>[2x]MSYKLTYFPIRGLAEPIRLVLVDQGIKFTDDRINASDWPSMKSHFHFGQLPCLYDGD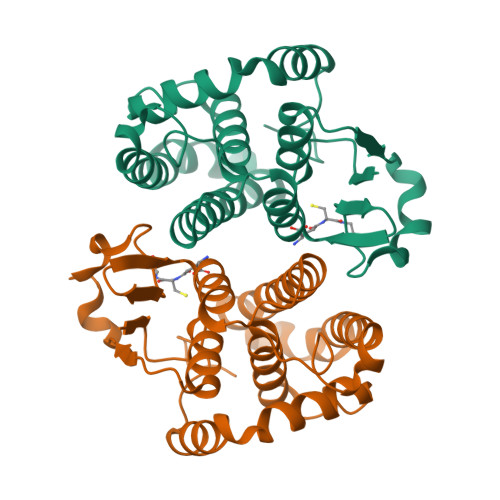HQIVQSGAILRHLARKHNLNGGNELETTHIDMFCEGVRDLHTKYTKMIYQAYDTEKDSYIKDILPVELAKFEKLLATRDDGKNFILGEKISYVDFVLFEELDIHQILDPHCLDKFPLLKAYHQRMEDRPGLKEYCKQRNRAKIPVNGNGKQ5-[3-(2-METHOXYPHENYL)-1H-PYRROLO[2,3-B]PYRIDIN-5-YL]-N,N-DIMETHYLPYRIDINE-3-CARBOXAMIDE 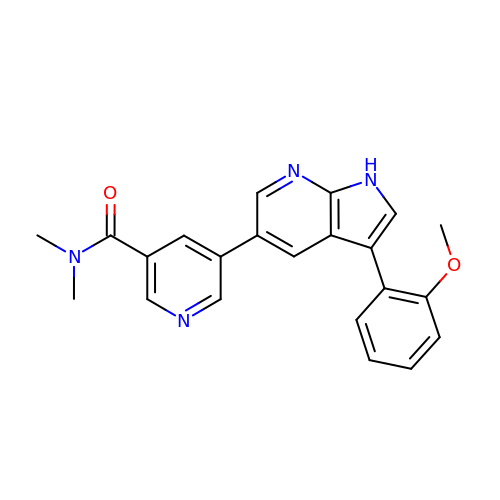| C22 H20 N4 O2 | GYQRHHQPEMOLKH-UHFFFAOYSA-N> MKVLCYGVRDVELPIFEACNKEFGYDIKCVPDYLNTKETAEMAAGFDAVILRGNCFANKQNLDIYKKLGVKYILTRTAGTDHIDKEYAKELGFPMAFVPRYSPNAIAELAVTQAMMLLRHTAYTTSRTAKKNFKVDAFMFSKEVRNCTVGVVGLGRIGRVAAQIF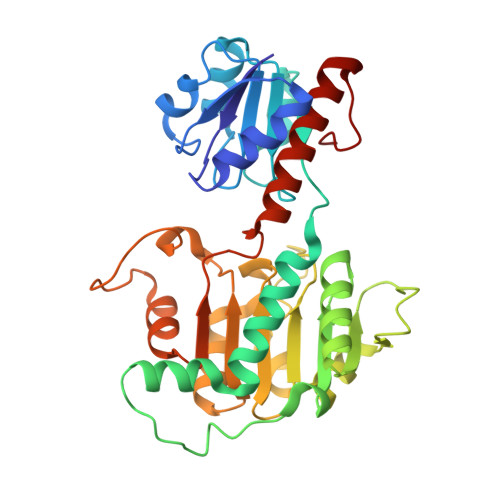HGMGATVIGEDVFEIKGIEDYCTQVSLDEVLEKSDIITIHAPYIKENGAVVTRDFLKKMKDGAILVNCARGQLVDTEAVIEAVESGKLGGYGCDVLDGEASVFGKDLEGQKLENPLFEKLVDLYPRVLITPHLGSYTDEAVKNMVEVSYQNLKDLAETGDCPNKIK>MGSKSFLTEQQIKILRLRARGLKQSEIAELLGTSRANISILERRALEKIEKARNIITIWEQINSKISVEVRKGEDIFTVPDKLFKKADELQIKVPYSTAEIIAFLVEHAPISDRIAKRDFTLFLDARDRLRISECLL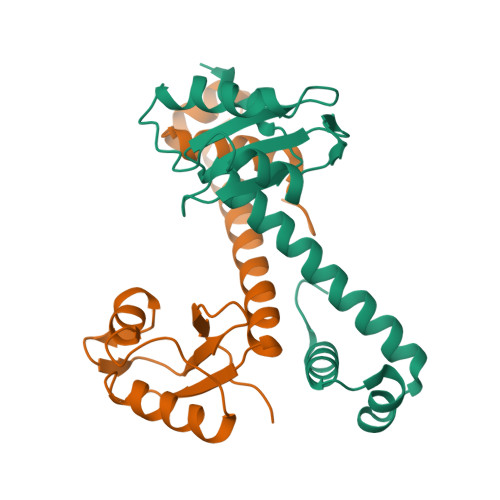EEFDEIGKQHHHHHH[2x]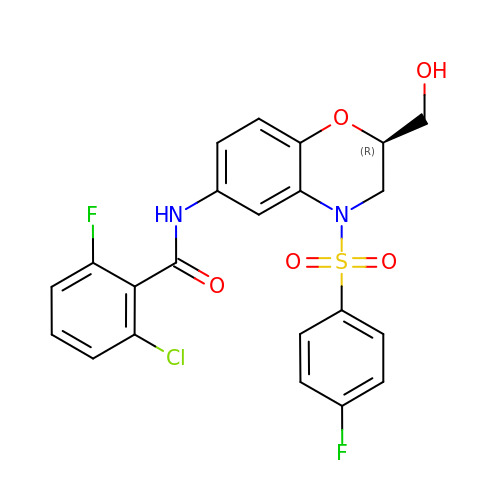2-chloranyl-6-fluoranyl-~{N}-[(2~{R})-4-(4-fluorophenyl)sulfonyl-2-(hydroxymethyl)-2,3-dihydro-1,4-benzoxazin-6-yl]benzamide | C22 H17 Cl F2 N2 O5 S | SLEGUDDXVCZXRA-OAHLLOKOSA-N> EDPQGDAAQKTDTSHHDQDHPTFNKITPNLAEFAFSLYRQLAHQSNSTNIFFSPVSIATAFAMLSLGTKADTHDEILEGLNFNLTEIPEAQIHEGFQELLRTLNQPDSQLQLTTGNGLFLSEGLKLVDKFLEDVKKLYHSEAFTVNFGDTEEAKKQINDYVEKGTQGKIVDLVKELDRDTVFALVNYIFFKGKWERPFEVKDTEEE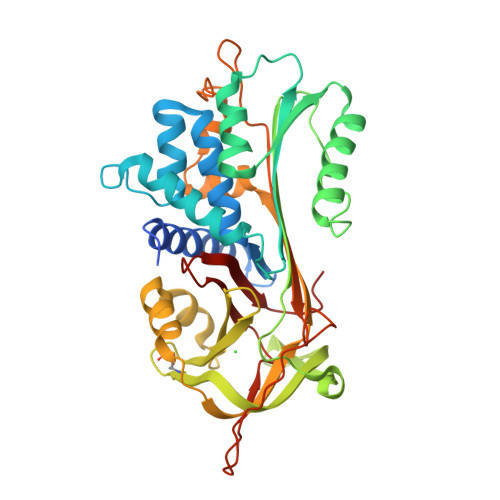DFHVDQVTTVKVPMMKRLGMFNIQHCKKLSSWVLLMKYLGNATAIFFLPDEGKLQHLENELTHDIITKFLENEDRRSASLHLPKLSITGTYDLKSVLGQLGITKVFSNGADLSGVTEEAPLKLSKAVHKAVLTIDEKGTEAAGAMFLEAIPMSIPPEVKFNKPFVFLMIEQNTKSPLFMGKVVNPTQK>[2x]GPLGSIMMMANNPEDWLSLLL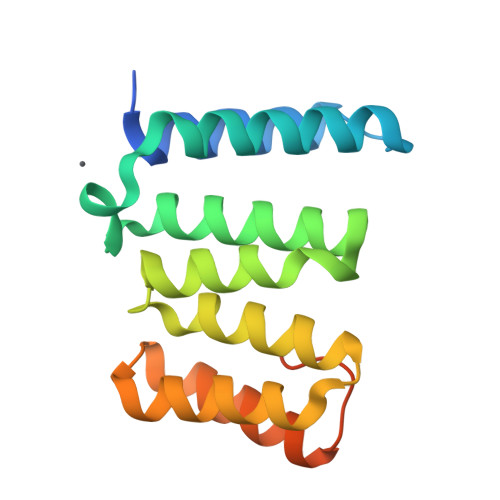KLEKNSVPLSDALLNKLIGRYSQAIEALPPDKYGQNESFARIQVRFAELKAIQEPDDARDYFQMARANCKKFAFVHISFAQFELSQGNVKKSKQLLQKAVERGAVPLEMLEIALRNLNLQKKQLLSEEEKKNLSASTVLT> DNGGYVPAVVIGTGYGAAVSALRLGEAGVQTLMLEMGQLWNQPGPDGNIFCGMLNPDKRSSWFKNRTEAPLGSFLWLDVVNR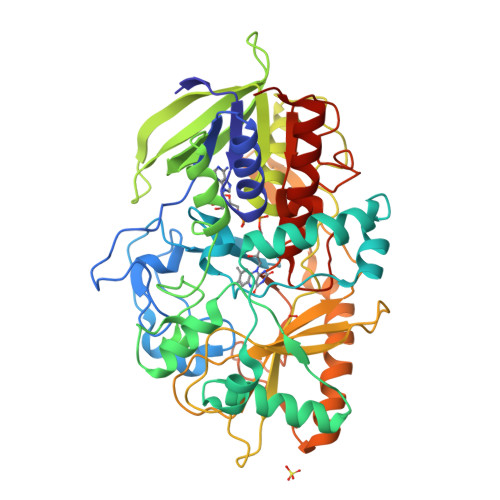NIDPYAGVLDRVNYDQMSVYVGRGVGGGSLVNGGMAVEPKRSYFEEILPRVDSSEMYDRYFPRANSMLRVNHIDTKWFEDTEWYKFARVSREQAGKAGLGTVFVPNVYDFGYMQREAAGEVPKSALATEVIYGNNHGKQSLDKTYLAAALGTGKVTIQTLHQVKTIRQTKDGGYALTVEQKDTDGKLLATKEISCRYLFLGAGSLGSTELLVRARDTGTLPNLNSEVGAGWGPNGNIMTARANHMWNPTGAHQSSIPALGIDAWDNSDSSVFAEIAPMPAGLETWVSLYLAITKNPQRGTFVYDAATDRAKLNWTRDQNAPAVNAAKALFDRINKANGTIYRYDLFGTQLKAFADDFCYHPLGGCVLGKATDDYGRVAGYKNLYVTDGSLIPGSVGVNPFVTITALAERNVERIIKQDVTAS(5S,8S,10R)-8-[(1R)-1-hydroxy-2-{[(5-propyl-1H-pyrazol-3-yl)methyl]amino}ethyl]-4,5,10-trimethyl-1-oxa-4,7-diazacyclohexadecane-3,6-dione | C25 H45 N5 O4 | 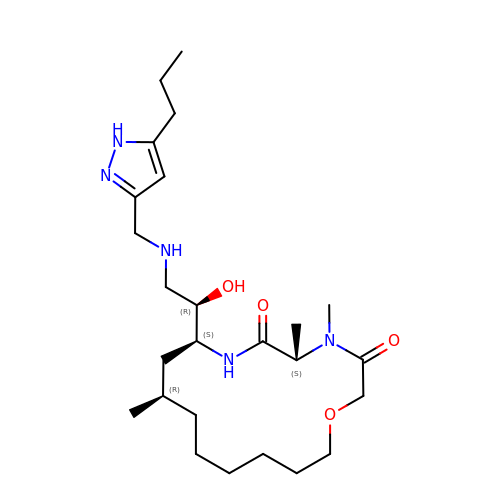NLWPKRWRLRUIHJ-CQIJRDABSA-N>[2x]M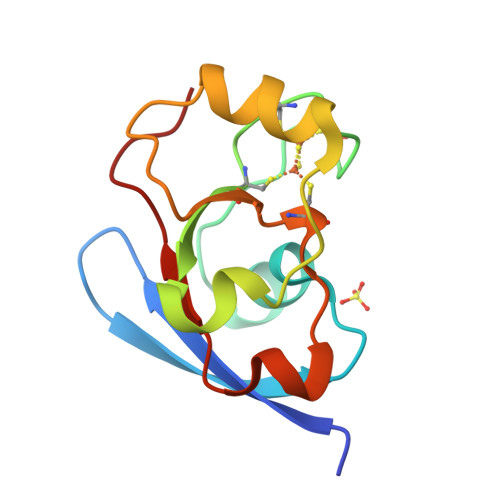ASDVVNVVFVDRSGQRIPVSGRVGDNVLHLAQRHGVDLEGACEASLACSTCHVYVSEDHLDLLPPPEEREDDMLDMAPLLQENSRLGCQIVLTPELEGAEFTLPKITR>[2x]MTMEQFLTSLDMIRSGCAPKFKLKTEDLDRLRVGDFNFPPSQDLMCYTKCVSLMAGSVNKKGEFNA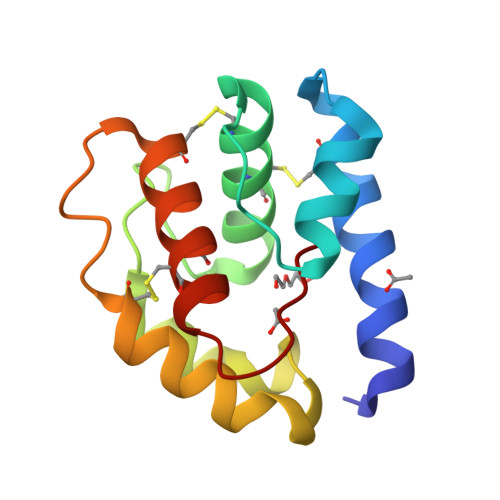PKALAQLPHLVPPEMMEMSRKSVEACRDTHKQFKESCERVYQTAKCFSENADGQFMWP> MIKSALLVLEDGTQFHGRAIGATGSAVGEVVFNTSMTGYQEILTDPSYSRQIVTLTYPHIGNVGTNDADEESSQVHAQGLVIRDLPLIASNFRNTEDLSSYLKRHNIVAIADIDTRKLTRLLREKGAQNGCIIAGDNPDAALALEKARAFPGLNGMDLAKEVTTAEAYSWTQGSWTLTGGLPQAKKEDELPFHVVAYDFGAKRNILRMLVDRGCRLTIVPAQTSAEDVLKMNPDGIFLSNGPGDPAPCDYAITAI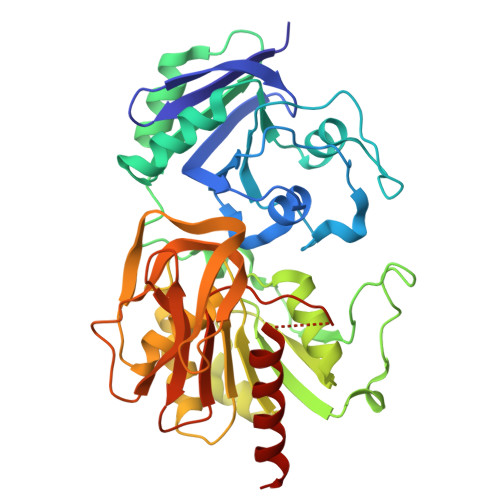QKFLETDIPVFGICLGHQLLALASGAKTVKMKFGHHGGNHPVKDVEKNVVMITAQNHGFAVDEATLPANLRVTHKSLFDGTLQGIHRTDKPAFSFQGHPEASPFPHDAAPLFDHFIELIEQYRKTAK>GPGSMSASAVNVTPGRNVVVVGTQWGDEGKGKIVDWLTDHAQGVVRFQGGHNAGHTLIIGGKKTILRLIPSGIMREGVACYIGNGVVLSPEALFKEIGELEEAGLSVRERLFISEATTLILPYHIAIDQAREARKGAGKIGTTGRGIGPAYEDKVGRRALRVQDLFDARTFADRLRENLDFHNFVLTQYLGGAAVDFQATLDTMLGYADRLRPMVADVSRRLYEENHAGRNLLFEGAQGTLLDIDHGTYPFVTSSNCVAGAAAAGAGVGPQKLNYILGITKAYCTRVGSGPFPSELYDADNPSRQDQIGITLANVGKEFGSVTGRPRRTGWLDAAALRRSIQINGVSGLCMTKLDVLDGLDEVKLCVGYKIDGEDADLLPRGAAEVARCEPVYETFGGWKESTVGINSWDALPA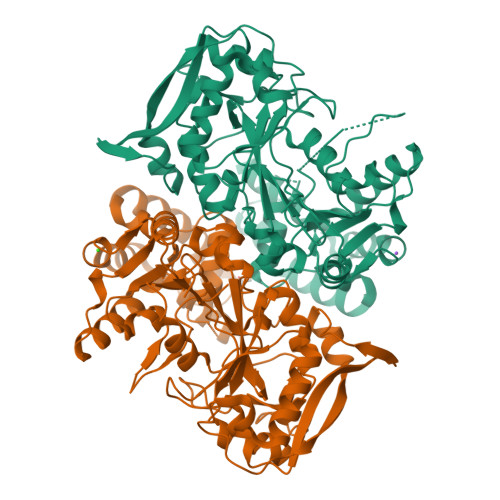NARAYLTRVQEVAGVPIDMVSTGPDRDETILLRHPFKV[4x]>SHMLRPVETPTREIKKLDGLWAFSLDRENCGIDQRWWESALQESRAIAVPGSFNDQFADADIRNYAGNVWYQREVFIPKGWAGQRIVLRFDAVTHYGKVWVNNQEVMEHQGGYTPFEADVTPYVIAGKSVRITVCVNNELNWQTIPPGMVITDENGKKKQSYFHDFFNYAGIHRSVMLYTTPNTWVDDITVVTHVAQDCNHASVDWQVVANGDVSVELRDADQQVVATGQGTSGTLQVVNPHLWQPGEGYLYELCVTAKSQTECDIYPLRVGIRSVAVKGEQFLINHKPFYFTGFGRHEDADLRGKGFDNVLMVHDHALMDWIGANSYRTSHYPYAEEMLDWADEHGIVVIDETAAVGFNLSLGIGF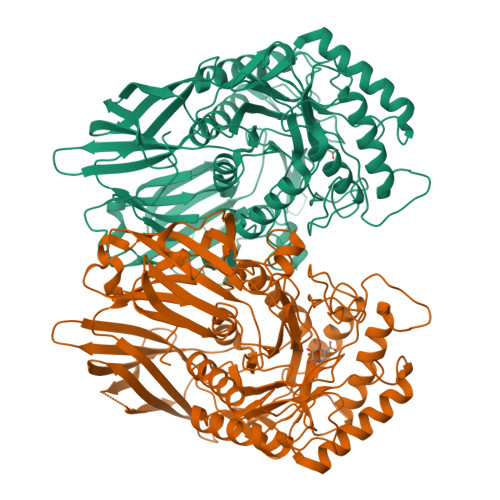EAGNKPKELYSEEAVNGETQQAHLQAIKELIARDKNHPSVVMWSIANEPDTRPQGAREYFAPLAEATRKLDPTRPITCVNVMFCDAHTDTISDLFDVLCLNRYYGWYVQSGDLETAEKVLEKELLAWQEKLHQPIIITEYGVDTLAGLHSMYTDMWSEEYQCAWLDMYHRVFDRVSAVVGEQVWNFADFATSQGILRVGGNKKGIFTRDRKPKSAAFLLQKRWTGMNFGEKPQQ[2x]>[2x]MEALVLVGHGTRLPYSKELLVKLAEKVKERNLFP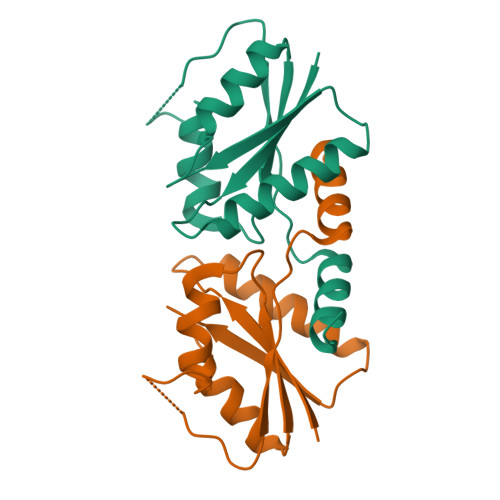IVEIGLMEFSEPTIPQAVKKAIEQGAKRIIVVPVFLAHGIHTTRDIPRLLGLIEDNHEHHHEHSHHHHHHHHHEHEKLEIPEDVEIIYREPIGADDRIVDIIIDRAFGR>GSHMGTEDLKYSLERLREILERLEENPSEKQIVEAIRAIVENNAQIVEAIRAIVEILALIVENNRAIIEALEAIGGGTKILEEMKKQLKDLKRALERG[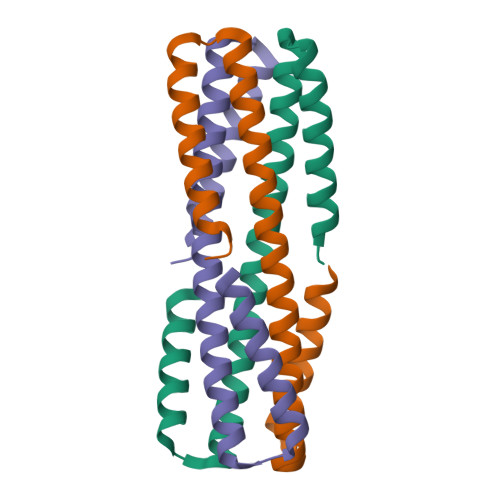3x]>[3x]QLTTESMPFNVAEGKEVLLLVHNLPQQLFGYSWYKGERVDGNRQIVGYAIGTQQATPGPANSGRETIYPNASLLIQNVTQNDTGFYTLQVIKSDLVNEEATGQFHVY

Like other hCEACAM family members, the hCEACAM1 IgV domain serves as the major ligand binding surface and is characterized by the presence of two anti-parallel β-sheets creating two distinct faces, the GFCC′ and ABED faces, respectively. The major mode of hCEACAM1 binding is homophilic such that it exists on the cell surface as collections of monomers and cis-dimers. hCEACAM1 has also been shown to form higher-order homo-oligomers and micro-clusters which, when present in a trans-configuration have been hypothesized to be important for strength of signal transduction. The structural basis for hCEACAM1 homo-oligomerization and the formation of higher-order structures is unknown.

To understand the structural basis for higher-order oligomerization and clustering of hCEACAM1, we solved the crystal structure of a tagless hCEACAM1 IgV domain at 2.2 Å resolution. Taken together, this oligomer crystal structure revealed simultaneous interactions through a primary (GFCC’-GFCC’) and secondary (ABED-ABED) contact at an atomic resolution level thus demonstrating the presence of two adhesion sites on a single hCEACAM1 IgV molecule. Notably, molecule (b) showed an additional interaction site involving the ABED surface with an interface area of 482.1 Å2 which was mediated by interactions with molecule (a) through residues located at its respective ABED face. This involved six hydrogen-bond interactions between the residues Q26-I67 (using nomenclature convention here and after, where Q26 residue is from molecule (b) and I67 residue in italics is from molecule (a)), Q27-Q76, Q53-Pro(P)59, S93-G63 and N23-Q54. The residues Q26 of molecule (b) and I67 of molecule (a) mediated two hydrogen-bond interactions and formed the central site for the formation of the ABED face, wherein the side-chain atoms NE2 and OE1 of molecule (b) residue Q26 made two hydrogen-bonds of 3.0 Å and 3.1 Å with the main chain oxygen and nitrogen atoms of molecule (a) residue I67, respectively. In contrast to the GFCC’ interface, the ABED interface did not involve hydrophobic interactions. Interestingly, molecule (b) residue S93, which is located within the FG loop, made a side-chain to backbone hydrogen-bond interaction of 2.8 Å through molecule (a) residue G63. Specifically, we observed that the GFCC’-based interface in this structure exhibited twice the area of the ABED interface. Consistent with the central role of GFCC’ face in dimerization and subsequent oligomerization, we observed GFCC’ face mediated interactions between two oligomers that enabled the formation of higher-order oligomers, wherein molecule (a) of the oligomer present in the crystal asymmetric unit mediated GFCC’ face interactions with a symmetry mate of molecule a (as) of the symmetry-related second oligomer. We therefore determined the crystallographic Debye-Waller factor (temperature factor or B factor) of all three molecules of the human CEACAM1 crystal structure reported here.> LMKLC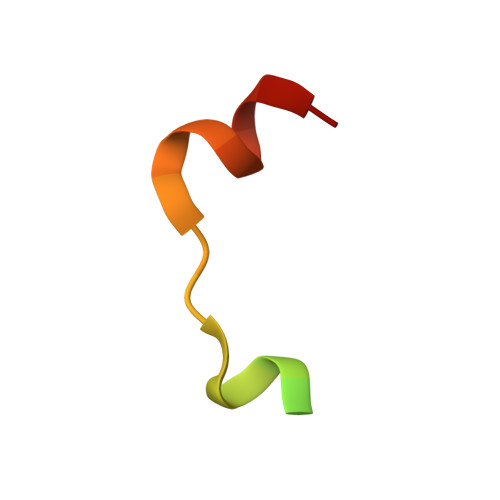GEVKPKNKARRRTTTQMELLYAD> MSRD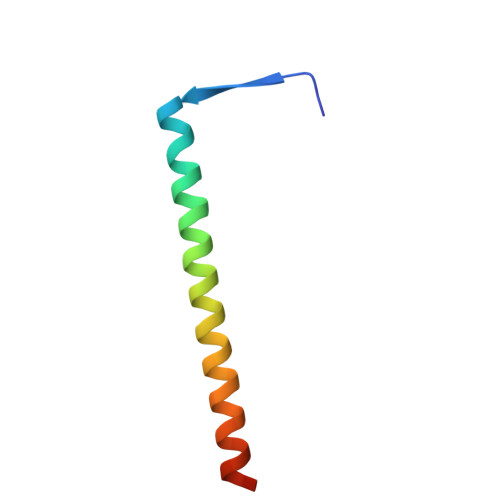LVTIPRDVWNDIQGYIDSLERENDSLKNQLMEADEYVAELEEKLNGTS>GSHMPNYDTSIDIEDIKKILPHRYPFLLVDKVIYMQPNKTIIGLKQVSTNEPFFNGHFPQKQIMPGVLQIEALAQLAG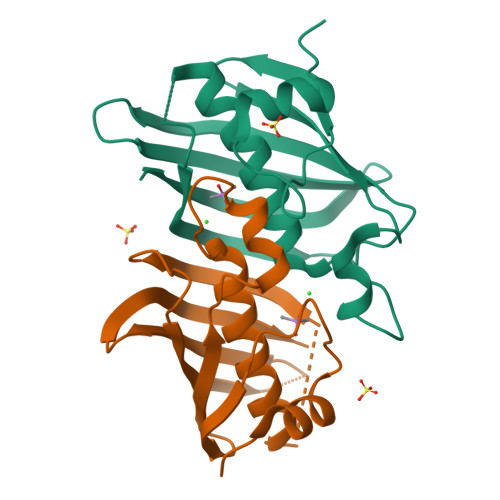ILCLKSDDSQKNNLFLFAGVDGVRWKKPVLPGDTLTMQANLISFKSSLGIAKLSGVGYVNGKVVINISEMTFALSK[6x]> XAA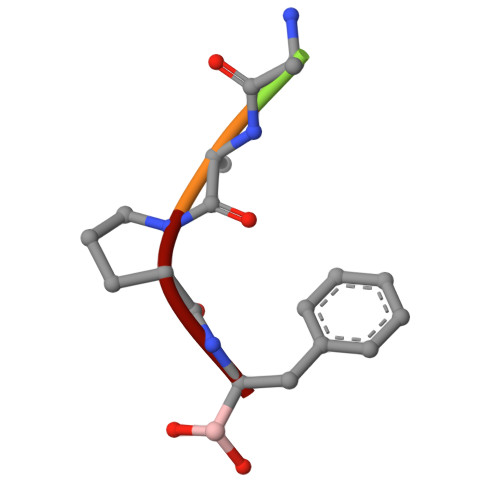PF> XAYHGAPHEIRNRYQHDRALEILDRQYSRDSYIYAHLVLYMKDSSLQIIRAQNPRIISRSYNWDQLVLPNYRINDEKYYGRSELRHLRDGLLSDNGGRSQHDKGMNEPVSFQFIVQGDVDLGSVWFRVNKYNNISSSSFAMEAVSERAENYIGPLMRPIRYFDREMAWSYVGKFDGILFPCHPVISFAVQRANRDGAGLYNGENIYKTLIRLNDSPDLYAHYDDEETSVANYWTRFQYLYRTKCDIAV

Cypoviruses, members of the family Reoviridae, subfamily Spinareovirus, possess a single capsid layer with turrets and are commonly embedded in crystalline occlusion bodies called polyhedra, which are formed in the cell cytoplasm and mainly composed of a single virus-encoded protein, polyhedrin. To ensure the delivery of virus particles to the target intestinal cells, allowing the transmission of packages of infectious virus between hosts by oral-faecal routes, polyhedra are disrupted only when they are exposed to the very alkaline pH environment found in insect midguts. The fold of all the polyhedrins is highly similar – a β-barrel core sitting on a base domain, surrounded by a common array of five helices (H1–H5). The strongest intermolecular interactions define a trimer composed of a cluster of three β-barrels sandwiched by helices top and bottom.

CPV19 possesses a combination of a long V1 and V2c hairpin. In CPV19, an extra V2c loop and elongated V1 eliminates the GTP space completely and displaces the ATP base ∼13 Å cf CPV1, to a site surrounded by V4 and V5. In CPV14 and CPV19 the V2n loops move to occupy some of the central space. The V5 regions of CPV5, 15, 17 and 19 differ, but all end in a similar place. In CPV1, 14, 15, 17, 18 and 20 solvent molecules can move between these two voids, whereas in CPV4, 5 and 19 they are blocked by tyrosine residues. CPV1, CPV19 and CPV20 were resistant such that only a small portion was dissolved in an hour while the other six cypovirus types plus the two deletion mutants dissolved dramatically. In fact the three CPVs (CPV1, 19 and 20) most resistant to alkali buffers all display more extensive interactions between the 3-fold symmetry-related subunits of the trimeric building block – strengthened by either pyridine binding (CPV1 and CPV20) or numerous protein–protein hydrogen bonds.3,3',3''-phosphanetriyltripropanoic acid | C9 H15 O6 P | 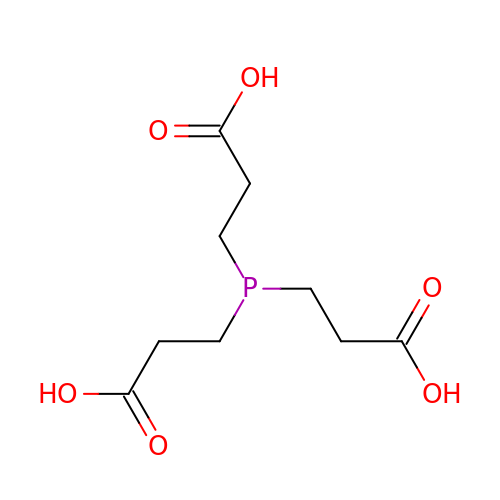PZBFGYYEXUXCOF-UHFFFAOYSA-N>MNQTLLSSFGTPFERVELALDALREGRGVMVLDDEDRENEGDMIFPAETMTVEQMALTIRHGSGIVCLCITEDRRKQLDLPMMVENNTSAYGTGFTVTIEAAEGVTTGVSAADRVTTVRAAIKDGAKPSDLNRPGHVFPLRAQAGGVLTRGGHTEATIDLMTLAGFKPAGVLCELTNDDGTMARAPECIAFAGQHNMAVVTIEDLVAY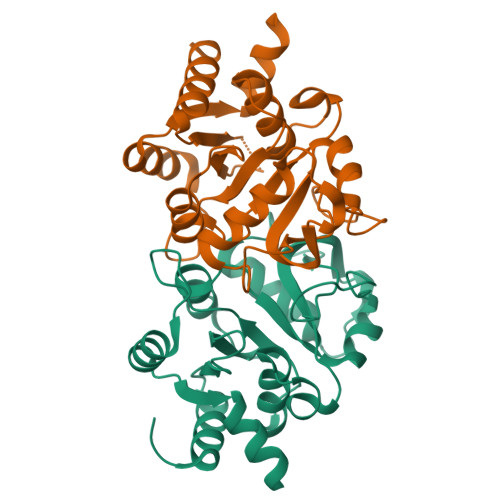RQAHERKAS[2x]4-(3-chloro-4-fluorophenyl)-5-(1,5-naphthyridin-2-yl)-1,3-thiazol-2-amine 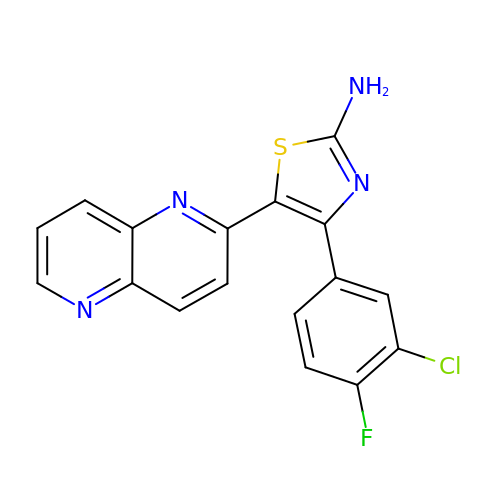| C17 H10 Cl F N4 S | QPTHMBUJLWRYEC-UHFFFAOYSA-N>SVFDSKFKGIHVYSEIGELESVLVHEPGREIDYITPARLDELLFSAILESHDARKEHKQFVAELKANDINVVELIDLVAETYDLASQEAKDKLIEEFLEDSEPVLSEEHKVVVRNFLKAKKTSRELVEIMMAGITKYDLGIEADHELIVDPMPNLYFTRDPFASVGNGVTIHYMRYKVRQRETLFSRFVFSNHPKLINTPWYYDPSLKLSIEGGDVFIYNNDTLVVGVSERTDLQTVTLLAKNIVANKECEFKRIVAINVPKWTNLMHLDTWLTMLDKDKFLYSPIANDVFKFWDYDLVNGGAEPQPVENGLPLEGLLQSIINKKPVLIPI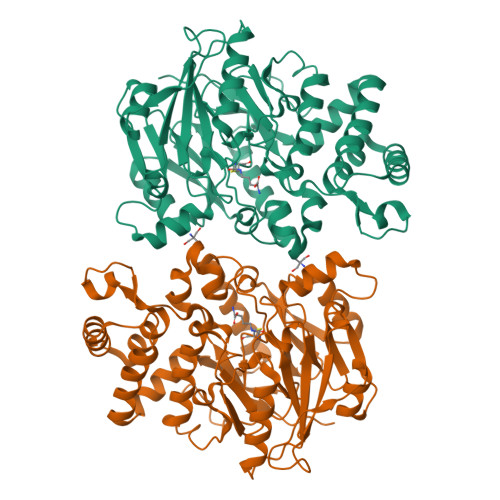AGEGASQMEIERETHFDGTNYLAIRPGVVIGYSRNEKTNAALEAAGIKVLPFHGNQLSLGMGNARCMSMPLSRKDVKW[2x]Cryptic unstable transcripts (CUTs) are rapidly degraded by the nuclear exosome in a process requiring the RNA helicase Mtr4 and specific adaptor complexes for RNA substrate recognition. The eleven-subunit MTREC comprises the zinc-finger protein Red1 and the Mtr4 homologue Mtl1. The zinc-finger protein Red1 serves as the main scaffold for the entire MTREC complex, assembling the individual submodules, including the Mtl1 helicase, into a large complex. Therefore, Red1 essentially acts as an adaptor between Mtl1 and the various MTREC submodules to provide a route for RNA substrates to the exosome through the unwinding activity of Mtl1.

Therefore, we switched to the Chaetomium thermophilum (ct) Mtr4–Red1 complex (homologues of spMtl1/spMtr4 and spRed1) due to superior biochemical properties of proteins and complexes from this thermophilic eukaryote. With these data at hand, we also succeeded in determining the structure of a complex comprising co-expressed (but not fused; split chain complex) ctMtr4SA and ctRed1pep, albeit at a lower resolution of 2.75 Å. Comparison of this structure with the single-chain structure revealed only small differences, as indicated by the low RMSD of 1.08 Å for Cα atoms of 273 residues, thus validating the single-chain structure. Notably, in our structure Red1 binds to both the KOW domain and stalk helices of the helicase. Importantly, in contrast to all previously characterized, canonical ligands Red1 utilizes a large interface that extends to the stalk helices and fixes them with respect to the KOW domain by inserting a U-shaped element that serves like a wedge. This extended binding interface observed for Red1 is supported by an extensive network of hydrophobic interactions and hydrogen bonds. However, replacing Ile1050 by an arginine (I1050R) completely abolished the interaction. Overall, the interaction of Mtr4 with Red1 described in our study shields the canonical adaptor protein-binding site, and suggests a mutually exclusive interaction of hMTR4 with either ZFC3H1 (the human Red1 homologue) or AIM-like motif containing adaptor proteins.

>MDEALIKDYHSIREQIDQYTKDMVLVMQHPTNCVKYINPGRLMHVVTSDGTDFGWGVIINFYERRPERNNPNPGWSPQESYVVEVLLRLSSDSGSVDSKLKDNQCIPAGIAPVTQKNDPGRWEVVPCLLSCMHGLSQIKLHVPDKKSGGSMDDPETRRRVGKSLLEVQRRFEDGIPHMDPIENMHIRDVEFKKLLRKIEVLESRLVANPLHNS[2x];>GAMALSYSSPLRFFRNFRFHPEFTRLVAGGWRSLTYSSRIDPDKEMCPYELEGTQCPSGCSFQHFVDITPAADERILLELSGSHHHHHH[2x]>MALSQATDPFRAAVEFTLMPMLITNPHLPDNPIVFANPAFLKLTGYEADEVMGRNSRFLQGHGTDPAHVRAIK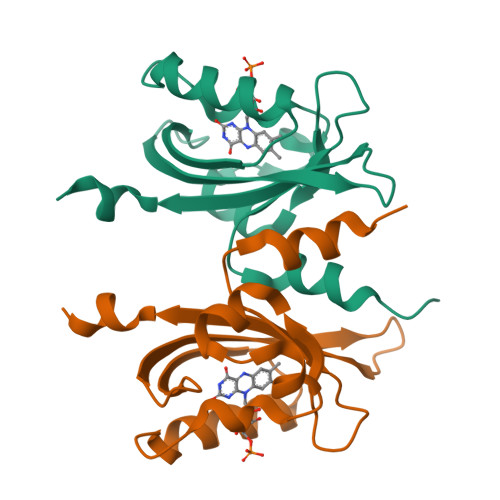SAIAAEKPIDIDIINYKKSGEAFWNRLHISPVHNANGRLQHFVSSQLDVTLELSRLVELEKERKTLSIEHHHHHH[4x]3-(2-imidazo[1,2-a]pyrazin-3-ylethynyl)-2-methyl-~{N}-[3-(4-methylpiperazin-1-yl)-5-(trifluoromethyl)phenyl]benzamide 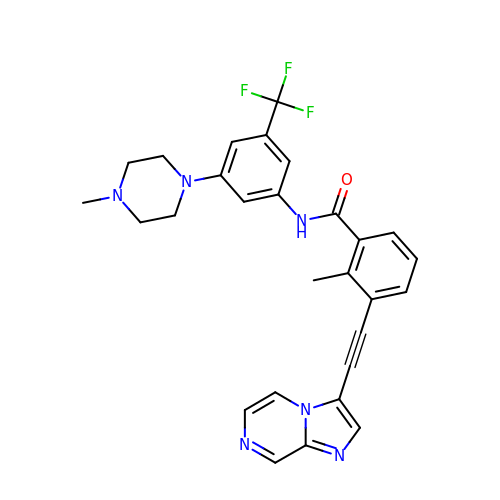| C28 H25 F3 N6 O | MFTCKIGOHVOPIP-UHFFFAOYSA-N The protein Eno1 (encoded by the ENO1 gene [C1_08500C_A]) plays a crucial role in the survival, pathogenicity, and antifungal drug susceptibilities of C. albicans. First, Eno1 has enolase activity and plays an essential role in glycolysis (catalyzing the conversion of 2-phospho-d-glycerate [2-PG] to phosphoenolpyruvate) in C. albicans, as knocking out the ENO1 gene renders C. albicans inviable on media with glucose as the sole carbon source. Second, Eno1 has transglutaminase activity and an ability to bind host plasminogen (PLG) and thus plays a key role in the invasion and virulence of C. albicans. Enolase is a dimeric enzyme and is critical for glycolysis, where it catalyzes the conversion of 2-PG to phosphoenolpyruvate.

To investigate the mechanism of action, we solved the crystal structure of C. albicans Eno1(CaEno1) and then compared the difference between this structure and that of Eno1 from humans. The diffraction data show that in an asymmetric unit, four Eno1 proteins form two dimers. The interface formed by the two dimers is through four pairs of hydrogen bonds, as follows: K80 in the B chain and E285 and R314 in the D chain form two hydrogen bonds, D72 in the B chain and Q286 in the D chain form one hydrogen bond, and S425 in the B chain forms one hydrogen bond with K202 in the D chain. Two CaEno1 molecules form a homodimer face-to-face in an antiparallel manner. In this dimer structure, the β1 to β3 strand plus the α5 helix and α16 helix of each Eno1 form an interaction interface. The β1 to β3 strand is exposed to the protein surface, and the rest of the β strands are embedded in the interior of Eno1. Interestingly the β4 to β13 strand forms a large β-barrel, while the α helices of the C-terminal domain are wrapped in the β-barrel to form a mixed α/β-barrel. This structure is similar to the three-dimensional structure of Eno1 in other species, suggesting that the active site of CaEno1 may also be in the C-terminal domain. We compared the sequence and structure of CaEno1 with S. cerevisiae Eno1 and hEno1. The consistency of amino acid sequences of CaEno1 versus S. cerevisiae Eno1 and CaEno1 versus hEno1 were 76.66% and 61.98%, respectively.

>MSYATKIHARYVYDSRGNPTVEVDFTTDKGLFRSIVPSGASTGVHEALELRDGDKSKWLGKGVLKAVANVNDIIAPALIKAKIDVVDQAKIDEFLLSLDGTPNKSKLGANAILGVSLAAANAAAAAQGIPLYKHIANISNAKKGKFVLPVPFQNVLNGGSHAGGALAFQEFMIAPTGVSTFSEALRIGSEVYHNLKSLTKKKYGQSAGNVGDEGGVAPDIKTPKEALDLIMDAIDKAGYKGKVGIAMDVASSEFYKDGKYDLDFKNPESDPSKWLSGPQLADLYEQLISEYPIVSIEDPFAEDDWDAWVHFFERVGDKIQIVGDDLTVTNPTRIKTAIEKKAANALLLKVNQIGTLTESIQAANDSYAAGWGVMVSHRSGETEDTFIADLSVGLRSGQIKTGAPARSERLAKLNQILRIEEELGSEAIYAGKDFQKASQLHHHHHH[4x]>[2x]SEFMTEPAIITNASDPAVQRIIDVTKHSRASIKTTLIEDTEPLMECIRAGVQFIEVYGSSGTPLDPALLDLCRQREIPVRLIDVSIVNQLFKAERKAKVFGIARVPRPARLADIAERGGDVVVLDGVKIVGNIGAIVRTSLALGAAGIVLVDSDLATIADRR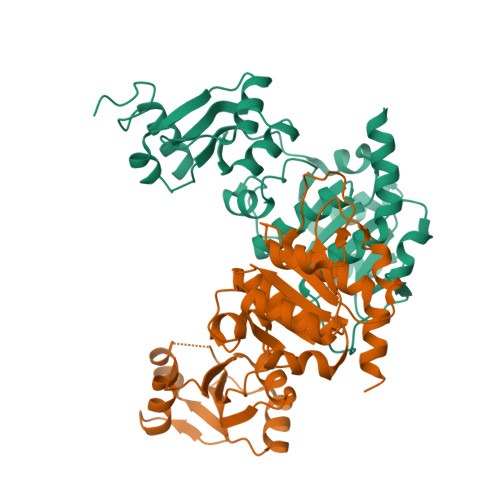LLRASRGYVFSLPVVLADREEAVSFLRDNDIALMVLDTDGDLGVKDLGDRADRMALVFGSEKGGPSGLFQEASAGTVSIPMLSSTESLNVSVSVGIALHERSARNFAVRRAAAQA> MAAVTGIALGMIETRGLVPAIEAADAMTKAAEVRLVGRQFVGGGYVTVLVRGETGAVNA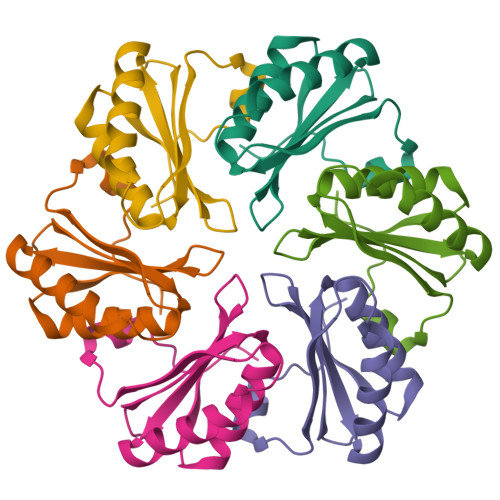AVRAGADACERVGDGLVAAHIIARVHSEVENILPKAPEA> MKVGQDKVVTIRYTLQVEGEVLDQGELSYLHGHRNLIPGLEEALEGREEGEAFQAHVPAEKAYGPHDPEGVQVVPLSAFPEDAEVVPGAQFYAQDMEGNPMPLTVVAVEGEEVTVDFNHPLAGKDLDFQVEVVKVREATPEELLHGH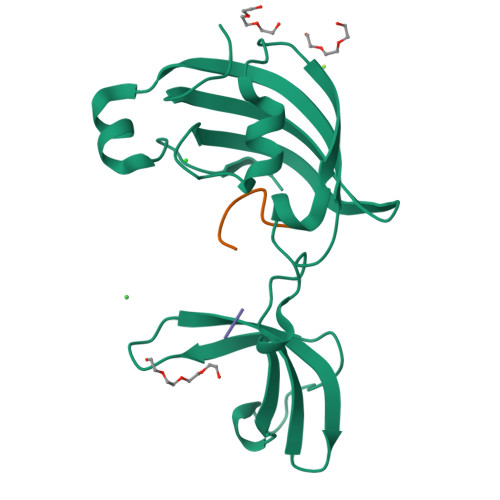AHPSGHHHHHH;> TRYWNAKALPFAFGA> MEDLIPLVNRLQDAFSAIGQNADLDLPQIAVVGGQSAGKSSVLENFVGRDFLPRGSGIVTRRPLVLQLVNSTTEYAEFLHCKGKKFTDFEEVRLEIEAETDRVTGTNKGISPVPINLRVYSPHVLNLTLVDLPGMTKVPVGDQPPDIEFQIRDMLMQFVTKENCLILAVSPANSDLANSDALKIAKEVDPQGQRTIGVITKLDLMDEGTDARDVLENKLLPLRRGYIGVVNRSQKDIDGKKDITAALAAERKFFLSHPSYRHLADRMGTPYLQKVLNQQLTNHIRDTLPGLRN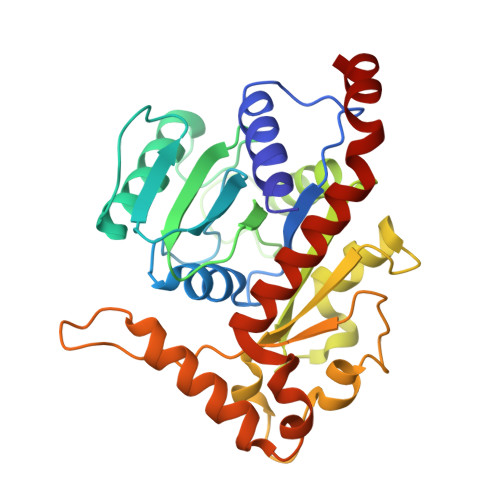KLQSQL> MEGLAGYVYKAASEGKVLTLAALLLNRSESDIRYLLGYVSQQGGQRSTPLIIAARNGHAKVVRLLLEHYRVQTQQTGTVRFDGYVIDGATALWCAAGAGHFEVVKLLVSHGANVNHTTVTNSTPLRAACFDGRLDIVKYLVENNANISIANKYDNTCLMIAAYKGHTDVVRYLLEQRADPNAKAHCGATALHFAAEAGHIDIVKELIKWRAAIVVNGHGMTPLKVAAESCKADVVELLLSHADCDRRSRIEALELLGASFANDRENYDIIKTYHYLYLAMLERFQDGDNILEKEVLPPIHAYGNRTECRNPQELESIRQDRDALHMEGLIVRERILGADNIDVSHPIIYRGAVYADNMEFEQCIKLWLHALHLRQKGNRNTHKDLLRFAQVFSQMIHLNETVKAPDIECVLRCSVLEIEQSMNRVKNISDADVHNAMDNYECNLYTFLYLVCISTKTQCSEEDQCKINKQIYNLIHLDPRTREGFTLLHLAVNSNTPVDDFHTNDVCSFPNALVTKLLLDCGAEVNAVDNEGNSALHIIVQYNRPISDFLTLHSIIISLVEAGAHTDMTNKQNKTPLDKSTTGVSEILLKTQMKMSLKCLAARAVRANDIN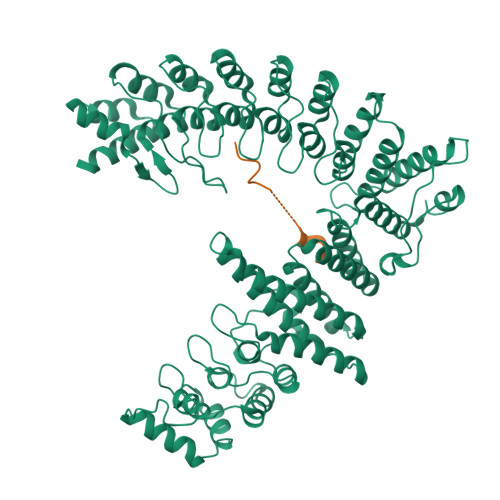YQDQIPRTLEEFVGFH;> GGGSGGGSKKHSLDLLSKERELNGKLRHLSP>MESEGEAGAKPVTALGAQVCQICGDGVGKTVDGEPFVACDVCAFPVCRPCYEYERKDGNQSCPQCKTRYKRHKGSPAILGDMEEDGAAAADASDFNYDSENQNQNQNQKQKISERMLSWQLTYPRGEEVGAPNYDKDVSHNHIPLLTSGQEVSGELSAASPERLSMASPAVGGGKRVHNIPYSSDINQSPNIRAGDPGLGNVAWKERVDGWKMKQEKNVVPMSTGQAASERGAGDIDASTDVLVDDSLLNDEARQPLSRKVSIPSSRINPYRMVIMLRLVILCIFLHYRITNPVPNAYPL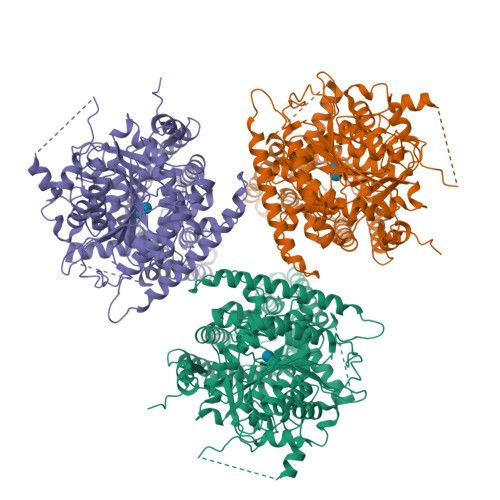WLVSVICEIWFAISWILDQFPKWLPVNRETYLDRLALRYDREGEPSQLAAVDIFVSTVDPLKEPPLVTANTVLSILAVDYPVDKVSCYVSDDGAAMLTFEALAETSEFARKWVPFSKKYSIEPRAPEWYFSQKIDYLKDKVHPSFVKDRRAMKREYEEFKVRINGLVSKAQKVPEEGWVMQDGTPWPGNNTRDHPGMIQVFLGQSGGLDTEGNELPRLVYVSREKRPGFQHHKKAGAMNALVRVSAVLTNGPFLLNLDCDHYINNSKALREAMCFMMDPNLGKHVCYVQFPQRFDGIDRNDRYANRNTVFFDINLRGLDGIQGPVYVGTGCVFNRTALYGYEPPLKPKHKKPGLLSSLCGGTRKKSSKSSKKGSDKKKSSKHVDPTVPIFNLEDIEEGVEGTGFDDEKSLLMSQMSLEKRFGQSAVFVASTLMENGGVPQSATPETLLKEAIHVISCGYEDKTDWGSEIGWIYGSVTEDILTGFKMHARGWRSIYCMPKRPAFKGSAPINLSDRLNQVLRWALGSVEILFSRHCPIWYGYGGRLKWLERFAYVNTTIYPVTAIPLLIYCILPAVCLLTNKFIIPQISNLASIWFISLFLSIFATGILEMRWSGVGIDEWWRNEQFWVIGGVSAHLFAVFQGLLKVLAGIDTNFTVTSKASDEDGDFAELYMFKWTTLLIPPTTLLIINLVGVVAGISYAINSGYQSWGPLFGKLFFAFWVIIHLYPFLKGLMGRQNRTPTIVVVWSVLLASIFSLLWVRIDPFTTRVTGPDVEECGINC[3x]>[2x]MITHRPRGIEHPYARSLDQLYPAIPIAGQSLTIGATTSGPCSRMRCFVLWPEHEQVFDMSPVNGTDSDAALLAGGEGHLAAAQQAALDADNGWQTSIPHLPDQDATYYFEALTLDGRTETSESFPLTPSHWSAEPVGHIDIDGDRFIPDSPLWLVSSAGTHRVKFALRIEGDEHVVGFGERYDQLDQRGLRLDSVVFEQYKAQGKHHRTYLPMPFAQVVNEAGRAWGFHVETTRRTWYDVAATV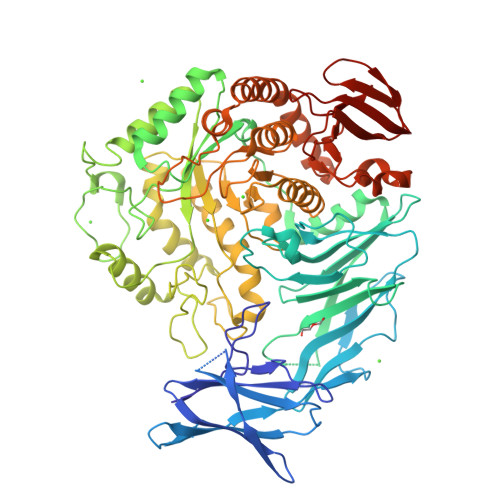SDRILIEVDLGFEAEKTPVVRVNTWSGSPTDVLNGFLDVAGRPAEMPEWIFGLWASGNEWNTQSLVMEQMDRHRNEGIPVSVVVIEAWSDEEGFTIFRDARYVPNQGQPHRGPDFTYPSDGAWPDPAGMIRELHERGIRVILWQIPLQKTDDDLGPEALAQGNALIASGHVVKEPDGTPYKNRGWWFPNALMPDLSTEAGRQWWTEQRRYLVEDLDIDGFKTDGGEHAWGSDLRYEDGRRGDEGNNLYPVNYARAYGDLLRSAGKYPVTFSRSGFTGSQAHGLYWAGDEDSTWEAFRSSITAGITAGACGILYWGWDLAGFSGPVPEAELYARAFAAATFMPIMQYHSEFHHHELPLRDRTPWNVAEQTGCGELIDLARHYTRVREALRPYLVAQTRQCLQTGKPLMRAMFYDHADDPEIWAHPRQYMLGDELLINPVTAPGATTWTTYLPEGQWEDYWSGEVSEGGHLVTRAVGWDIIPVYRRVGAAL>SNAMALKPTIYKFRIALSDMNNDYYDSKNLT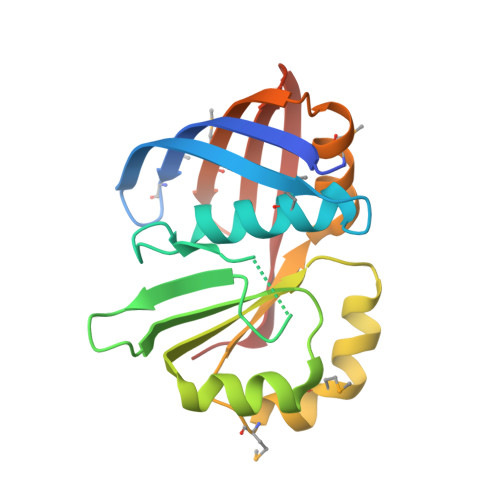IALHPSEKPQRMLARILAFCLNAQKDLEFTKGLSTTEEPDLWHVADDQSITHWIEIGEPEPDRIKKASRLAKQVKVYTYNTKAPVWWEKMSGKFSMLPVSVESFDYDAIDMICQHLDRGTNLSVMITGTSIFVDVNDQHVEVTVKELQSHDAP[4x]> MMKIVPPKPFFFEAGERAVLLLHGFTGNSADVRMLGRFLESKGYTCHAPIYKGHGVPPEELVHTGPDDWWQDVMNGYEFLKNKGYE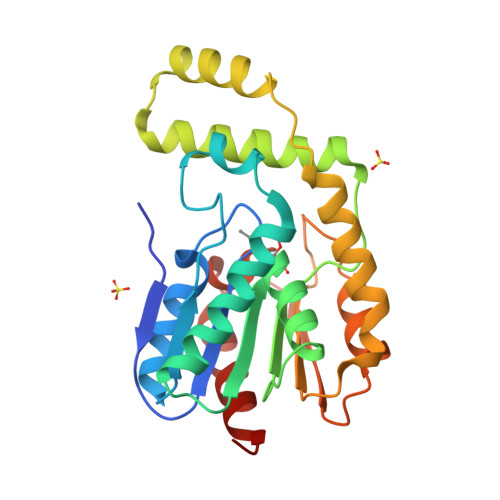KIAVAGLSLGGVFSLKLGYTVPIEGIVTMCAPMYIKSEETMYEGVLEYAREYKKREGKSEEQIEQEMEKFKQTPMKTLKALQELIADVRDHLDLIYAPTFVVQARHDEMINPDSANIIYNEIESPVKQIKWYEQSGHVITLDQEKDQLHEDIYAFLESLDW> GPGSEFELMQGGSSTNHETAGLRTEMLSRLFTAATSISHFEEAH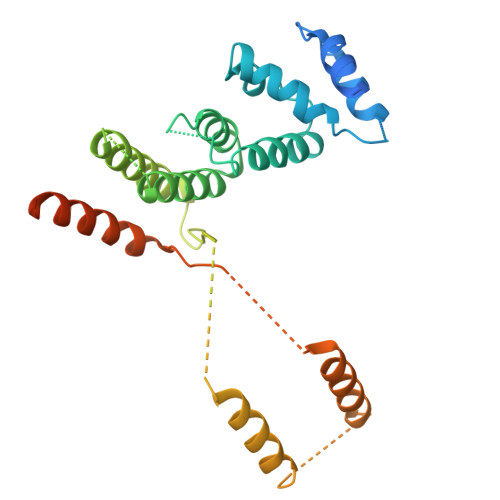SALLSMDDEAMQKSYLRRLVEKMCETGQSSELITLPFSGLQTKVDDILVEKCRATRDVLNGVPYHQILYAWRINHNDYRGGAAILLDRLQKLRRAGEGDKVIANEHGNEDALDTQVTRQYLLLINALSCVPPQEAYILEDVLPGDGRGGDDADGDRNGGKAGDDLEADIDELEKKLDVEGGADAAKGDEMAAEEDAALIEKMKRFSTRNGQNLPARRLLMLADLRKQYQQELDRIVAIQNNQFGFGAEDDLMDLAGGSGHHHHHHHHHH> MAAPVVAPPGVVVSRANKRSGAGPGGSGGGGARGAEEEPPPPLQAVLVADSFDRRFFPISKDQPRVLLPLANVALIDYTLEFLTATGVQETFVFCCWKAAQIKEHLLKSKWCRPTSLNVVRIITSELYRSLGDVLRDVDAKALVRSDFLLVYGDVISNINITRALEEHRLRRKLEKNVSVMTMIFKESSPSHPTRCHEDNVVVAVDSTTNRVLHFQKTQGLRRFAFPLSLFQGSSDGVEVRYDLLDCHISICSPQVAQLFTDNFDYQTRDDFVRGLLVNEEILGNQIHMHVTAKEYGARVSNLHMYSAVCADVIRRWVYPLTPEANFTDSTTQSCTHSRHNIYRGPEVSLGHGSILEENVLLGSGTVIGSNCFITNSVIGPGCHI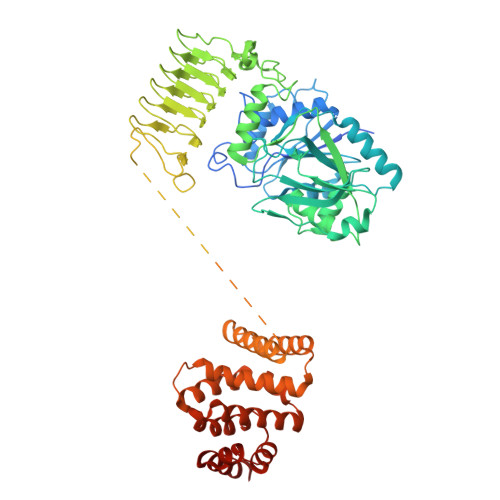GDNVVLDQTYLWQGVRVAAGAQIHQSLLCDNAEVKERVTLKPRSVLTSQVVVGPNITLPEGSVISLHPPDAEEDEDDGEFSDDSGADQEKDKVKMKGYNPAEVGAAGKGYLWKAAGMNMEEEEELQQNLWGLKINMEEESESESEQSMDSEEPDSRGGSPQMDDIKVFQNEVLGTLQKGKEENISCDNLVLEINSLKYAYNISLKEVMQVLSHVVLEFPLQQMDSPLDSSRYCALLLPLLKAWSPVFRNYIKRAADHLEALAAIEDFFLEHEALGISMAKVLMAFYQLEILAGETILSWFSQRDTTDKGQQLRKNQQLQRFIQWLKEAEEESSEDD> MEFLNSIPWEEVVPGQFTANPGFQVTDYFEIVRQPADGNCFYHSIAEL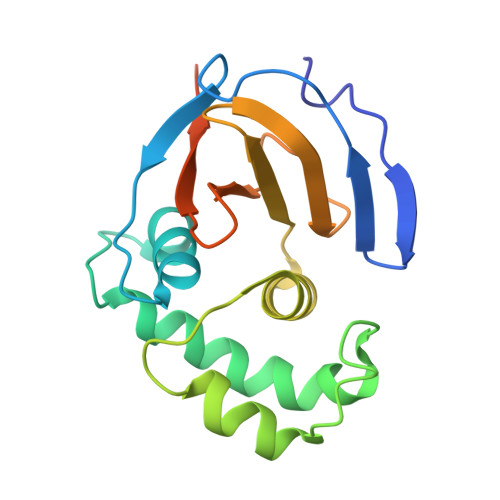FVPNKNDFSFRLVKQHLELAARRFFEEESEAKGLGLSLEKYLEVAMCDNEWGGSLEASMLAKHLDITIVIWVIEGPSRVAAAVKFGPGDVAGAINLLHTGYNHFDALRLLVDDSQVSRQPRSGSHHHHHH>MSNHTYRVIEIVGTSPDGVDAAIQGGLARAAQTMRALDWFEVQSIRGHLVDGAVAHFQVTMKVGFRLEDS[16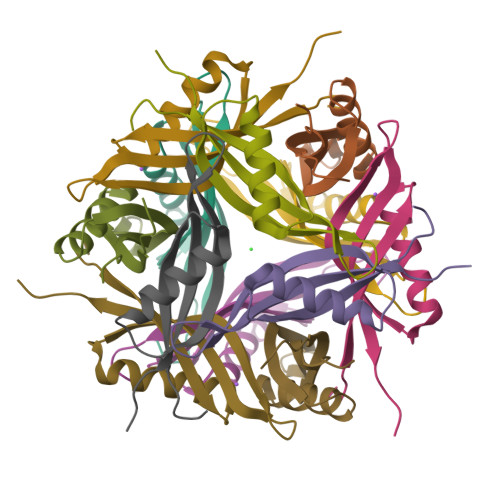x]methyl 4-(azepan-1-yl)-3-[(4-methoxyphenyl)sulfonylamino]benzoate | C21 H26 N2 O5 S 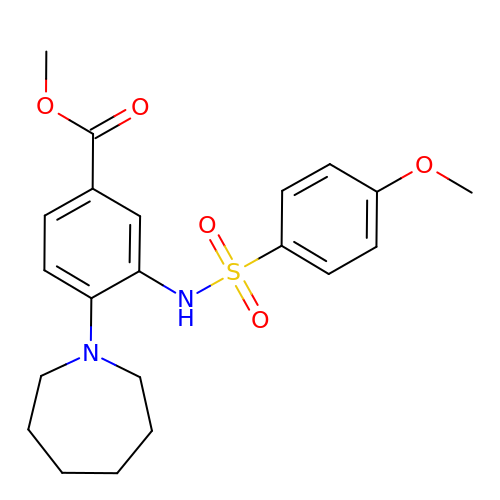| KUHNIQWJBKIEFH-UHFFFAOYSA-N AcrIF24 is a recently identified Acr that inhibits the type I-F CRISPR-Cas system. Interestingly, AcrIF24 was predicted to be a dual-function Acr and Aca. Aca proteins are transcriptional regulators which commonly inhibit the expression of acr genes by forming an acr-aca operon. AcrIF24 is dimeric and binds a short inverted repeat sequence in the acrIF23-acrIF24 operon promoter to repress acr expression.

The purified AcrIF24 protein sample was successfully crystallized and diffracted to 2.5 Å. The crystal belongs to space group P6522 with one molecule present in the asymmetric unit. The final structural model contains the complete AcrIF24 sequence (residues M1 to S228). The overall shape of the AcrIF24 structure resembled a bird and was composed of three distinct domains. The wing domain was formed by five β-sheets (β1–β5) and one long α-helix (α1) at the N-terminal part of AcrIF24, while the body domain was composed of six α-helixes (α3-α8) forming a helical bundle fold at the C-terminus of AcrIF24. The head domain was formed by four β-sheets (β6–β9) and one α-helix (α2) was localized between the wing and body domains. Because the electrostatic surface features are sometimes important for predicting the function of a protein, we analyzed the electrostatic surface features of AcrIF24. This analysis showed that AcrIF24 contained a highly positively charged cleft in the bottom part of the body domain, although negatively and positively charged surfaces were evenly dispersed in the AcrIF24 structure. B-factor analysis showed that most of the head domain had relatively higher B-factors (average 88.25 Å2), indicating that the head domain might be flexible. PPI analysis showed that the complex formation significance score (CSS) of the MolA/Sym1 dimer was 0.2 (the score ranges from 0 to 1 as the relevance of the interface to complex formation increases), while that of the MolA/Sym2 dimer was 0, indicating that the MolA/Sym1 dimer might be the biologically relevant form. However, our intact, fully folded crystal structure of AcrIF24 indicates that AcrIF24 can be in ordered conformation without binding to Cascade.

> MNAIHIGPFSITPAARGLHYGGLPHHQWTLYYGPREMAIKTLPDSYTSSEVRDEFSDIIAEFVIDARHRYAPDVLELVNSDGDAVLARVAVSRLPEALSGCIPDDRFPYWLLTASRPRLGLPVTLNEYTALAVELSAPPLAWITGLLPGEVLTHDAEEWRPPTSWELRHVVGEGSFTGVSGAAAAALLGMSATNFRKYTAGDSAANRQKISFAAWHYLLDRLGVKRASLEHHHHHH> ASQDQVDDLLDSLG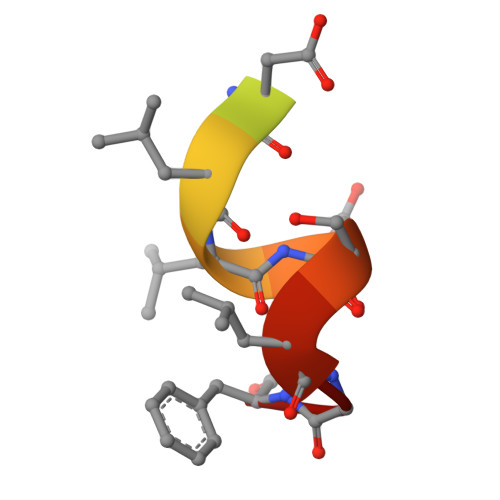F>[2x]QKVGKFSPEVHPPITWQECADDGSCKTMNGEIVIDANWRWVHSEQGTNCYTGNTWNPTLCPDDKTCAENCYLDGANYESVYGITTEDDSVRLNFITQSQGKNIGSRTFLMANSTNYQMFYVLGQEFSFDVDVSNLDCGLNGALYLVSMDSDGGIARFPSNEAGAQYGTGYCDAQCPRDLKFISGSAN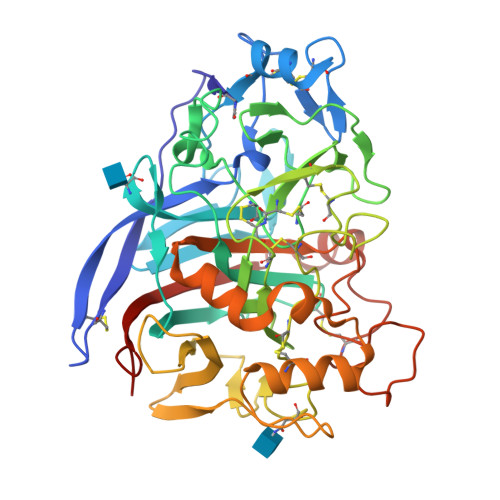VEGWIPSSNNPNTGYGNHGSCCAEMDLWEANNMATALTPHPCDTSSQTVCESDSCGGATSSNRYGGLCDPDGCDYNPYRMGNTTFFGPGQTVDTKSVMTVVTQFITNDGTTTGTLKSIKRLYVQNGQVISQSESTVPGVAGNEITEDFCHNQKQVFGDKDSFTKHGGLAAMGDALKNGMVLVLSLWDDYLADMLWLDSNYPTTSPVTEPGVARGPCSTSSGTPTDVESKYPNAYVVYSNIKVGPINSTFKNN> FRISLICFPKAGCEEITRQGRRVVLKPQEYFAQ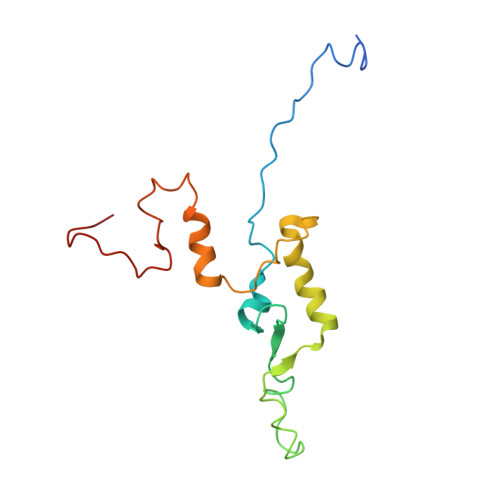HRMQVWQMRFKEMGPPFSRVWVALGGKMRRRRIGRQIDVKDMRYYWRPIEPQYQRLYMSRLRIKDHSNKRVQPMRLRATNNDIGQASSLKEWERSSDRKYGAALAPPKKRDFEFRVF>MNQNLLVTKRDGSTERINLDKIHRVLDWAAEGLHNVSISQVELRSHIQFYDGIKTSDIHETIIKAAADLISRDAPDYQYLAARLAIFHLRKKAYGQFEPPALYDHVVKMVEMGKYDNHLLEDYTEEEFKQMDTFIDHDRDMTFSYAAVKQLEGKYLVQNRVTGEIYESAQFLYILVAACLFSNYPRETRLQYVKRFYDAVSTFKISLPTPIMSGVRTPTRQFSSCVLIECGDSLDSINATSSAIVKYVSQRAGIGINAGRIRALGSPIRGGEAFHTGCIPFYKHFQTAVKSCSQGGVRGGAATLFYPMWHLEVESLLVLKNNRGVEGNRVRHMDYGVQINKLMYTRLLKGEDITLFSPSDVPGLYDAFFADQEEFERLYTKYEKDDSIRKQRVKAVELFSLMMQERASTGRIYIQNVDHCNTHSPFDPAIAPVRQSNLCLQIALPTKPLNDVNDENGEIALCTLSAFNLGAINNLDELEELAILAVRALDALLDYQDYPIPAAKRGAMGRRTLGIGVINFAYYLAKHGKRYSD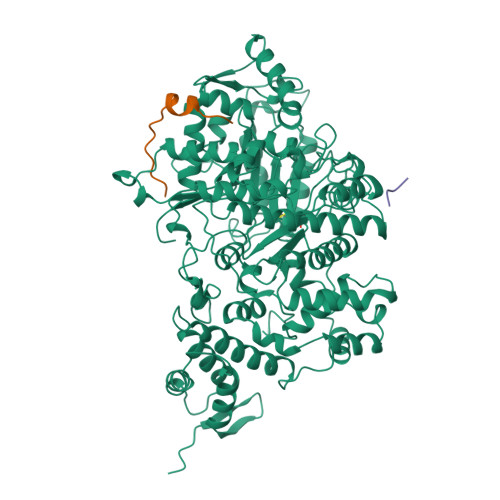GSANNLTHKTFEAIQYYLLKASNELAKEQGACPWFNETTYAKGILPIDTYKKDLDTIANEPLHYDWEALRESIKTHGLRNSTLSALMPSETSSQISNATNGIEPPRGYVSIKASKDGILRQVVPDYEHLHDAYELLWEMPGNDGYLQLVGIMQKFIDQSISANTNYDPSRFPSGKVPMQQLLKDLLTAYKFGVKTLYYQNTRDGAEDAQDDLVPSIQDDGCESGACKI[3x];>[4x]YLVGQIDSEVDTDDLSNFQL>LPRETDEEPEEPGKTGSFVEMVDNLRGKSGQGYYVEMTVGSPPQTLNILVDTGSSNFAVGAAPHPFLHRYYQRQLSSTYRDLRKGVYVPYTQGKWEGELGTDLVSIPHGPNVTVRANIAAITESDKFFINGSNWEGILGLAYAEIARPDDSLEPFFDSLVKQTHVPNLFSLQLCGAGFPLNQSEVLASVGGSMIIGGIDHSLYTGSLWYTPIRREWYYEVIIVRVEINGQDLKMDCKEYNYDKSIVDSGTTNLRLPKKVFEAAVKSIKAASSTEKFPDGFWLGEQLVCWQAGTTPWNIFPVISLYLMGEVTNQSFRITILPQQYLRPVEDVATSQDDCYKFAISQSSTGTVMG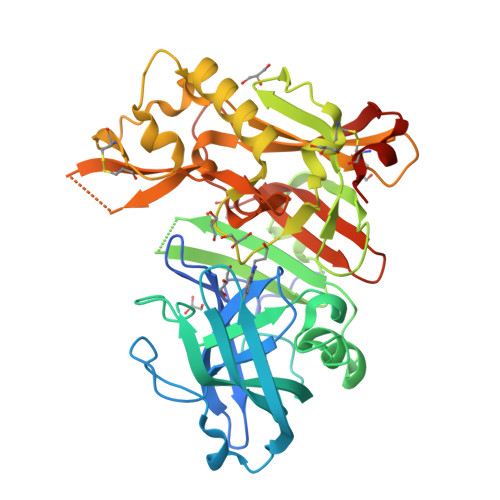AVIMEGFYVVFDRARKRIGFAVSACHVHDEFRTAAVEGPFVTLDMEDCGYNIPQTDES[3x]>SITENTSWNKEFSAEAVNGVFVLCKSSSKSCATNDLARASKEYLPASTFKIPNAIIGLETGVIKNEHQVFKWDGKPRAMKQWERDLTLRGAIQVSAVPVFQQIAREVGEVRMQKYLKKFSYGNQNISGGIDKFWLEGQLRISAVNQVEFLESLYLNKLSASKENQLIVKEALVTEAAPEYLVHSKTGFSGVGTESNPGVAWWVGWVEKETEVYFFAFNMDIDNESKLPLRKSIPTKIMESEGIIGG[3x];> SITENTSWNK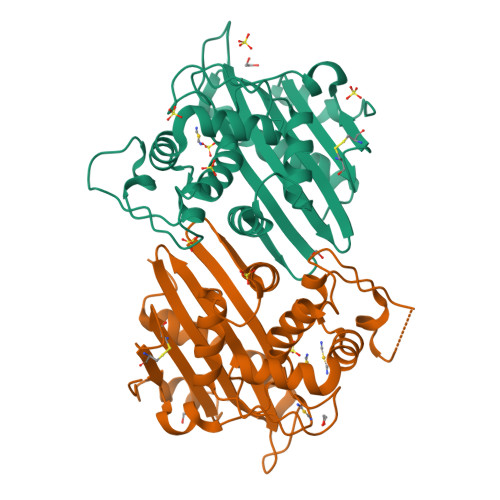EFSAEAVNGVFVLCKSSSKSCATNDLARASKEYLPASTFKIPNAIIGLETGVIKNEHQVFKWPGKPRAMKQWERDLTLRGAIQVSAVPVFQQIAREVGEVRMQKYLKKFSYGNQNISGGIDKFWLEGQLRISAVNQVEFLESLYLNKLSASKENQLIVKEALVTEAAPEYLVHSKTGFSGVGTESNPGVAWWVGWVEKETEVYFFAFNMDIDNESKLPLRKSIPTKIMESEGIIGG>GSHMEVVNKGDYYSIQGKYDEIIVANKHYPLSKDYNPGENPTAKAELVKLIKAMQEAGFPISDHYSGFRSYETQTKLYQDYVNQDGKEAADRYSARPGYSEHQTGLAFDVIGTDGDLVTEEKAAQWLLDHAADYGFVVRYLKGKEKETGYMAEEWHLRYVGKEAKEIAESGLSLEEYYGFEGGDYVD[5x]

We report biochemical properties and crystal structures of the LD-carboxypeptidases LdcB from Streptococcus pneumoniae, Bacillus anthracis, and Bacillus subtilis. The enzymes are active against bacterial cell wall tetrapeptides and adopt a zinc-carboxypeptidase fold characteristic of the LAS superfamily. LD-carboxypeptidases subsequently hydrolyze the L-Lys[A2pm]—D-Ala bond to release the tripeptide. The LdcB enzymes are single domain proteins comprising two subdomains separated by a V-shaped cleft.

Despite attempting to crystallise LdcB enzymes with a range of synthetic ligands, one crystal structure was obtained, that of SpLdcB in complex with MurNAc—L-Ala—D-γ-Gln—L-Lys—(D-Asn). This ligand is a close chemical analog of the true reaction product, as it contains half of the repeating unit of the glycan component of PG and comprises a tripeptide stem peptide that is branched at the L-lysine, the location of the crosslink position in natural PG. There are six molecules of SpLdcB in this crystallographic asymmetric unit, though none of the interfaces represent a stable multimeric form. Residual electron density was retained throughout refinement in only one of the five molecules, chain A, into which MurNAc—L-Ala—D-γ-Gln—L-Lys—(D-Asn) could be built and refined unambiguously. First, the MurNAc moiety is situated at the very top of the intersubdomain cavity and makes little contact with the protein. The Cα and Cβ atoms of L-alanine at position 1 of the peptide pack against the face of Tyr144, a conserved amino acid in many LdcB sequences, to discriminate against the D-stereoisomer in this subsite, S3. The NH2 group of the D-γ-Gln of position 2 is located in subsite S2, 2.3 Å away from and in hydrogen bonding distance of Glu204, an invariant amino acid in LdcB sequences. As expected of a reaction product complex, the lysine carboxylate is located adjacent to the active site zinc in subsite S1. One of the carboxylic oxygens completes the zinc tetrahedral geometry with His153/Asp160/His207, and the second oxygen forms a salt bridge with Arg120, which is either arginine or lysine in LdcB orthologs. Most of these residues (Asp167 to Glu171) move by 10–15 Å in the presence of ligand to open up the cleft by refolding into an additional turn at the N terminus of α-helix 4.> REVLTGGHSVSAPQENRIYVMDSVFMHLTESRVHVYDYTNGKFLGMVPTAFNGHVQVSNDGKKIYTMTTYHERITRGKRSDVVEVWDADKLTFEKEISLPPKRVQGLNYDGLFRQTTDGKFIVLQNASPATSIGIVDVAKGDYVEDVTAAAGCWSVIPQPNRPRSFMTICGDGGLLTINLGEDGKVASQSRSKQMFSVKDDPIFIAPALDKDKAHFVSYYGNVYSADFSGDEVKVDGPWSLLNDEDKAKNWVPGGYNLVGLHRASGRMYVFMHPDGKEGTHKFPAAEIWVMDTKTKQRVARIPGRDALSMTIDQQRNLMLTLDGGNVNVYDISQPEPKLLRTIEGAAEASLQV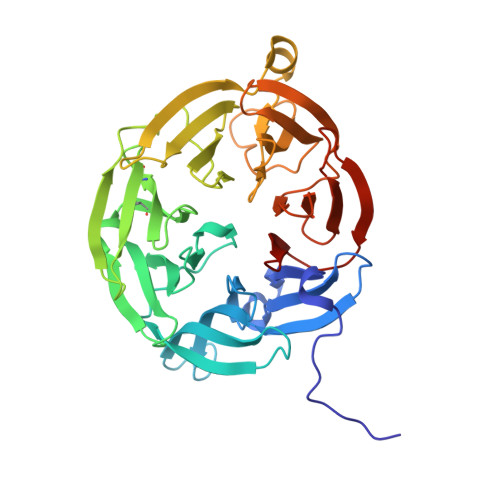QFHPVGGT> GATGRTTIAIDPVTRIEGHLKAEVVVENGKVVDARLSGGMYRGFETILRGRDPRDASQIVQRICGVCPTAHSTASVLALDEAFGAKVPNNGRITRNLIFGANYLQSHILHFYHLSAQDFVQGPDTAPFVPRFPKSDLRLSKELNKAGVDQYIEALEVRRICHEMVALFGGRMPHVQGQVVGGATEIPTKEKLVEYAARFKKVRDFVEQKYVPVVYTIGSKYKDMFKVGQGFKAALCVGAFPLDNSGKKHLFMPGVYAKGKDMPFDPSKIKEYVKYSWFAEETTGLNYKEGKTIPAPDKAGAYSFVKAPRYDGLSLEVGPLARMWVNNPELSPVGKKLLKDLFGISAKKFRDLGEEAAFSLMGRHVARAEETYYMLGAIEGWLKEIKAGEDTVVMPAVPAS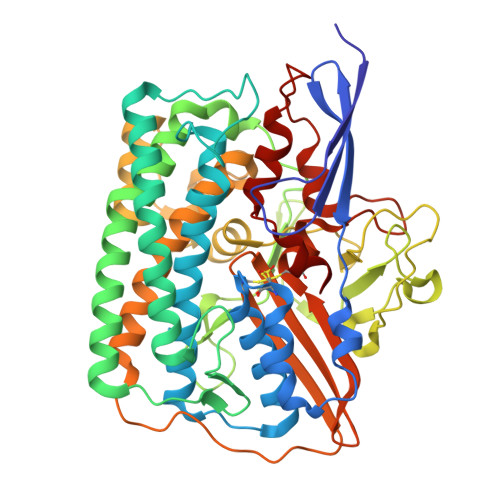AEGTGFTEAPRGSLLHYVKVKDSKIDNYQIVSASLWNCNPRDDMGQRGAVEEALIGIPVDDIQNPVNVARLIRAFDPULSCAVH> SIESTSKSNFQKLSRGNIDVLKGRGSISSTRQRAIYPYFEAANADEQQPLFFYIKKDRFDNHGYDQYFYDNTVGPNGIPTL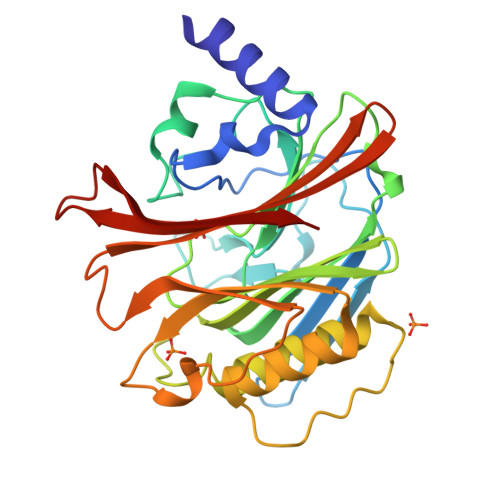NTYTGEIPSDSSSLGSTYWKKYNLTNETSIIRVSNSARGANGIKIALEEVQEGKPVIITSGNLSGCTTIVARKEGYIYKVHTGTTKSLAGFTSTTGVKKAVEVLELLTKEPIPRVEGIMSNDFLVDYLSENFEDSLITYSSSEKKPDSQITIIRDNVSVFPYFLDNIPEHGFGTSATVLVRVDGNVVVRSLSESYSLNADASEISVLKVFSKKF> MKHHHHHHHHHHGTSAGLEVLFQGPGNAIKLIHFLFRHKIIKFKTEIINFHEAYQQFVTIYEQYDDMVQEYLEIRTLLQLIQIKITNAQQRILDIEQKLSLATDHQKEFSQSLLQLKKPIEANLQMAEKSKAGLEEKLSGLKTRLPSCIERFNKFMTQIEINDIKTLIRLLGDEVADRGSCDYFTLRILDFLYQNQIAIKIILSNHGYEFIHAYEKLVVGQPFKPKGYIGDIQIKSFWGLQLLLEQSVITEEELRSLVERAYKPTLKIIDYSLSEDGITLYSHAPIRFDSIRMAASQLGVTYNDSTKEALAETIDQLNAQLQIYMKNNMLHLLFENNEINDPTNMTDEERNASPLIYLVWNRWNESKEVENARPGKYNGYFVTYVHGHDPFQSPLTYVYNLDTL

Here we describe the crystal structure and biochemical properties of WipA (or IcmW-interacting protein A; lpg2718), an effector protein originally identified because of its dependence on the IcmSW complex for translocation, but for which the function is unknown. The crystal structure reveals a two-domain structure comprising a metallophosphoesterase attached to an 85-Å-long α-helical hairpin forming a coiled-coil at its tip. Although WipA exhibits a serine/threonine phosphatase fold, it functions preferentially as a protein-tyrosine phosphatase (PTP), even though there are no structural similarities to the general PTP fold. The protein forms homodimers in solution, and the dimer is mediated by the tip of the helical hairpin domain.

The protein, however, degraded into shorter fragments, the most prominent of which had a molecular mass of 46 kDa. Mass spectrometry analysis of this fragment yielded a sequence coverage that included amino acids at the N and C termini from residue 34 to residue 411. A construct of this core domain (termed “WipA411”) was therefore produced, expressed, purified, and crystallized, yielding crystals diffracting to 1.84 Å resolution. Its structure was determined using the single-wavelength anomalous dispersion method applied to selenomethionine (SeMet)-substituted crystals of WipA411. Residues including nine residues of the N-terminal His tag linker and the protein sequence up to residue 410 were visible in the electron density and were therefore included in the final model. The WipA411 crystals contain one molecule/asymmetric unit (AU) and no metal. The first is between the tip of the α-helical hairpin of one molecule and the globular domain from a symmetry-related molecule and is observed in both the WipA411 and WipA435 structures (and interaction details in B). This interface includes five H-bonds and one salt bridge covering a surface area of ∼550 Å2. Overall, all proteins including the shorter WipA411 elute as dimers.>RTYPVEIAGVRRELPIVQVGPGVAVALLNLLGDTELTEAAAEALAKRLPPEVEVLVTPEVKAVPLAHALSRITGKPYVVARKTEKPYMINPVSRQVLSITTGKPQLLVLDGADIPRVRGKKVAIVDDVVSTGSTLAGLRELI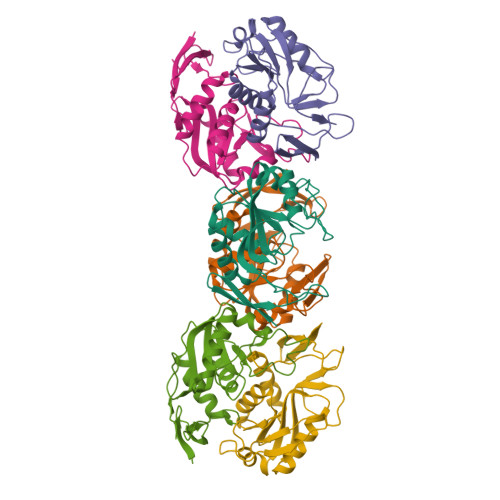ESVGGEVVAVLAVFTEGTPRQDVVALGHLPLF[6x]> EPRSVAVFPWHS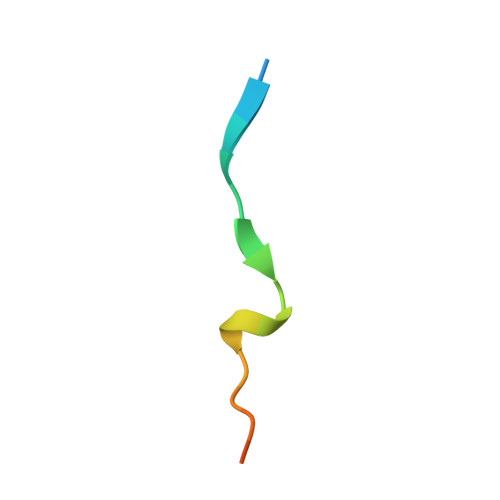LVPFLAPSQ>KDFVRPKLVTIIRSGVKPRKAVRVLLNKKTAHSFEQVLTDITEAIKLETGVVKKLY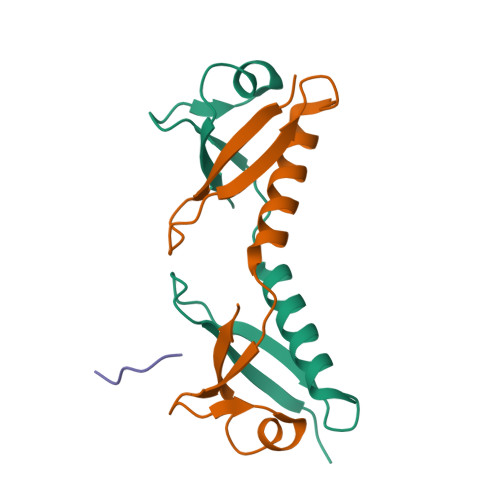TLDGKQVTCLHDFFGDDDVFIACGP[4x];>PESSEG[3x]>VPMGKFAMYPDWQPDADFIRLAALWGVALREPVTTEELASFIAYWQAEGKVF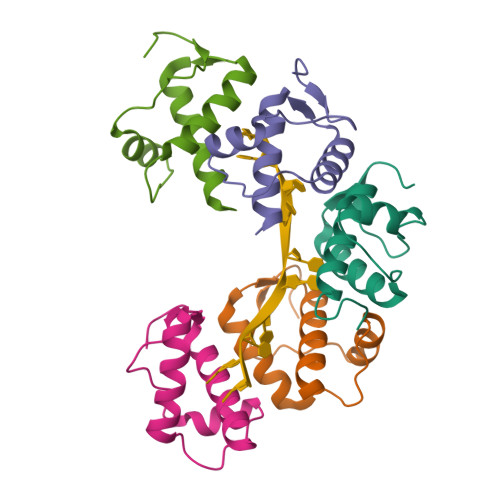HHVQWQQKLARSLQIGRASNGGLP[5x]6-[{(2S)-2-AMINO-3-[4-(BENZYLOXY)PHENYL]PROPYL}(HYDROXY)AMINO]-6-OXOHEXANOIC 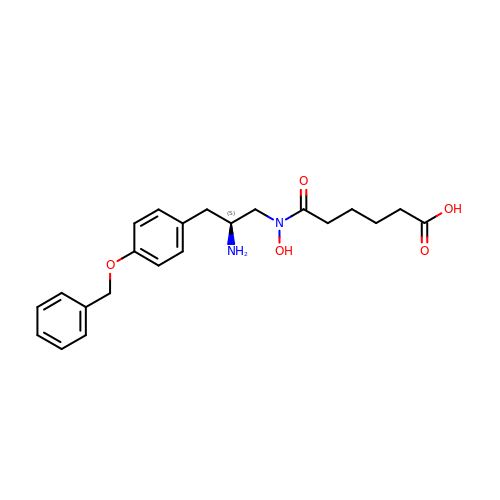ACID) | C22 H28 N2 O5 | YOYHDDAKAGRLRC-IBGZPJMESA-N> MNHPFGKEEAASQKQLFGFFCECLRRGEWELAQACVPQLQEGQGDIPKRVEDILQALVVCPNLLRCGQDINPQRVAWVWLLVLEKWLAREKKLLPVVFRRKLEFLLLSEDLQGDIPENILEELYETLTQGAVGHVPDGNPRRESWTPRLSSEAVSVLWDLLRQSPQPAQALLELLLEEDDGTGLCHWPLQNALVDLIRKALRALQGPDSVPPGVVDAIYGALRTLRCPAEPLGVELHLLCEELLEACRTEGSPLREERLLSCLLHKASRGLLSLYGHTYAEKVTEKPPRATASGKVSPDHLDPERAMLALFSNPNPAEAWKVAYFYCLSNNKHFLEQILVTALTLLKEEDFPNLGCLLDREFRPLSCLLVLLGWTHCQSLESAKRLLQTLHRTQGPGCDELLRDACDGLWAHLEVLEWCIQQSSNPIPKRDLLYHLHGGDSHSVLYTLHHLTNLPALREEDVLKLLQKVPAKDPQQEPDAVDAPVPEHLSQCQNLTLYQGFCAMKYAIYALCVNSHQHSQCQDCKDSLSEDLASATEPANDSLSSPGAANLFSTYLARCQQYLCSIPDSLCLELLENIFSLLLITSADLHPEPHLPEDYAEDDDIEGKSPSGLRSPSESPQHIAHPERKSERGSLGVPKTLAYTMPSHVKAEPKDSYPGPHRHSFLDLKHFTSGISGFLADEFAIGAFLRLLQEQLDEISSRSPPEKPKQESQSCSGSRDGLQSRLHRLSKVVSEAQWRHKVVTSNHRSEEQPSRRYQPATRHPSLRRGRRTRRSQADGRDRGSNPSLESTSSELSTSTSEGSLSAMSGRNELHSRLHPHPQSSLIPMMFSPPESLLASCILRGNFAEAHQVLFTFNLKSSPSSGELMFMERYQEVIQELAQVEHKIENQNSDAGSSTIRRTGSGRSTLQAIGSAAAAGMVFYSISDVTDKLLNTSGDPIPMLQEDFWISTALVEPTAPLREVLEDLSPPAMAAFDLACSQCQLWKTCKQLLETAERRLNSSLERRGRRIDHVLLNADGIRGFPVVLQQISKSLNYLLMSASQTKSESVEEKGGGPPRCSITELLQMCWPSLSEDCVASHTTLSQQLDQVLQSLREALELPEPRTPPLSSLVEQAAQKAPEAEAHPVQIQTQLLQKNLGKQTPSGSRQMDYLGTFFSYCSTLAAVLLQSLSSEPDHVEVKVGNPFVLLQQSSSQLVSHLLFERQVPPERLAALLAQENLSLSVPQVIVSCCCEPLALCSSRQSQQTSSLLTRLGTLAQLHASHCLDDLPLSTPSSPRTTENPTLERKPYSSPRDSSLPALTSSALAFLKSRSKLLATVACLGASPRLKVSKPSLSWKELRGRREVPLAAEQVARECERLLEQFPLFEAFLL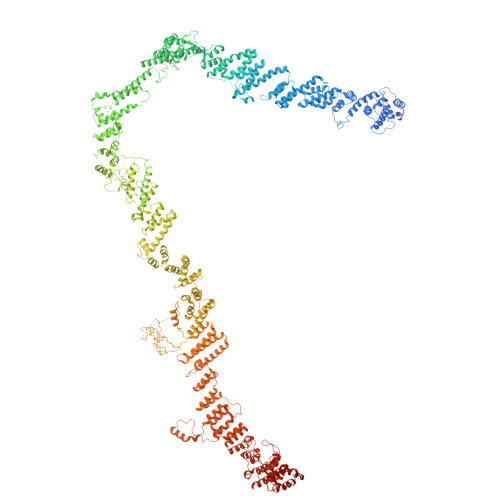AAWEPLRGSLQQGQSLAVNLCGWASLSTVLLGLHSPIALDVLSEAFEESLVARDWSRALQLTEVYGRDVDDLSSIKDAVLSCAVACDKEGWQYLFPVKDASLRSRLALQFVDRWPLESCLEILAYCISDTAVQEGLKCELQRKLAELQVYQKILGLQSPPVWCDWQTLRSCCVEDPSTVMNMILEAQEYELCEEWGCLYPIPREHLISLHQKHLLHLLERRDHDKALQLLRRIPDPTMCLEVTEQSLDQHTSLATSHFLANYLTTHFYGQLTAVRHREIQALYVGSKILLTLPEQHRASYSHLSSNPLFMLEQLLMNMKVDWATVAVQTLQQLLVGQEIGFTMDEVDSLLSRYAEKALDFPYPQREKRSDSVIHLQEIVHQAADPETLPRSPSAEFSPAAPPGISSIHSPSLRERSFPPTQPSQEFVPPATPPARHQWVPDETESICMVCCREHFTMFNRRHHCRRCGRLVCSSCSTKKMVVEGCRENPARVCDQCYSYCNKDVPEEPSEKPEALDSSKNESPPYSFVVRVPKADEVEWILDLKEEENELVRSEFYYEQAPSASLCIAILNLHRDSIACGHQLIEHCCRLSKGLTNPEVDAGLLTDIMKQLLFSAKMMFVKAGQSQDLALCDSYISKVDVLNILVAAAYRHVPSLDQILQPAAVTRLRNQLLEAEYYQLGVEVSTKTGLDTTGAWHAWGMACLKAGNLTAAREKFSRCLKPPFDLNQLNHGSRLVQDVVEYLESTVRPFVSLQDDDYFATLRELEATLRTQSLSLAVIPEGKIMNNTYYQECLFYLHNYSTNLAIISFYVRHSCLREALLHLLNKESPPEVFIEGIFQPSYKSGKLHTLENLLESIDPTLESWGKYLIAACQHLQKKNYYHILYELQQFMKDQVRAAMTCIRFFSHKAKSYTELGEKLSWLLKAKDHLKIYLQETSRSSGRKKTTFFRKKMTAADVSRHMNTLQLQMEVTRFLHRCESAGTSQITTLPLPTLFGNNHMKMDVACKVMLGGKNVEDGFGIAFRVLQDFQLDAAMTYCRAARQLVEKEKYSEIQQLLKCVSESGMAAKSDGDTILLNCLEAFKRIPPQELEGLIQAIHNDDNKVRAYLICCKLRSAYLIAVKQEHSRATALVQQVQQAAKSSGDAVVQDICAQWLLTSHPRGAHGPGSRK>NQPYRTGFHFQPPKNWMNDPNGPMIYKGIYHLFYQWNPKGAVWGNIVWAHSTSTDLINWDPHPPAIFPSAPFDINGCWSGSATILPNGKPVILYTGIDPKNQQVQNIAEPKNLSDPYLREWKKSPLNPLMAPDAVNGINASSFRDPTTAWLGQDKKWRVIIGSKIHRRGLAITYTSKDFLKWEKSPEPLHYDDGSGMWECPDFFPVTRFGSNGVETSSFGEPNEILKHVLKISLDDTKHDYYTIGTYDRVKDKFVPDNGFKMDGTAPRYDYGKYYASKTFFDSAKNRRILWGWTNESSSVEDDVEKGWSGIQTIPRKIWLDRSGKQLIQWPVREVERLRTKQVKNLRNKVLKSGSRLEVYGVTAAQADVEVLFKVRDLEKADVIEPSWTDPQLICSKMNVSVKSGLGPFGLMVLASKNLEEYTSVYFRIFKARQNSNKYVVLMCSDQSRSSLKEDNDKTTYGAFVDINPHQPLSLRALIDHSVVESFGGKGRACITSRVYPKLAIGKSSHLFAFNYGYQSVDVLNLNAWSMNSAQIS[6x];>[6x]GANNLVETTCKNTPNYQLCLKTLLSDKRSATGDITTLA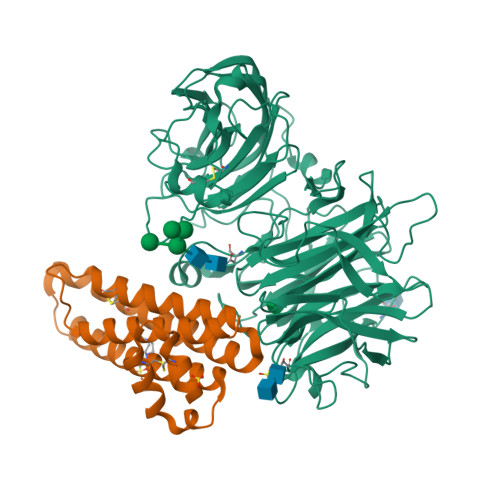LIMVDAIKAKANQAAVTISKLRHSNPPAAWKGPLKNCAFSYKVILTASLPEAIEALTKGDPKFAEDGMVGSSGDAQECEEYFKGSKSPFSALNIAVHELSDVGRAIVRNLL> EDLLKNL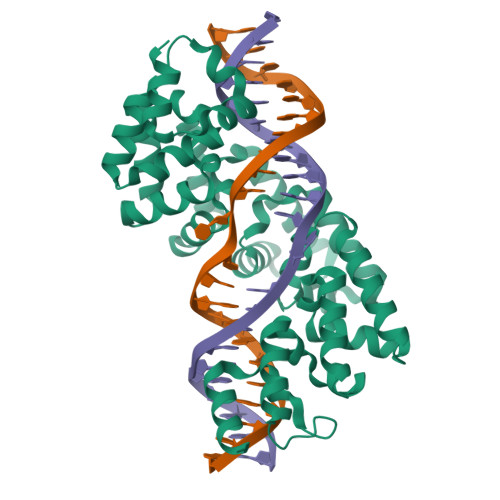LTMGVDIDMARKRQPGVFHRMITNEQDLKMFLLSKGASKEVIASIISRYPRAITRTPENLSKRWDLWRKIVTSDLEIVNILEASPESFFRSNNNLNLENNIKFLYSVGLTRKCLCRLLTNAPRTFSNSLDLNKQMVEFLQAAGLSLGHNDPADFVRKIIFKNPFILIQSTKRVKANIEFLRSTFNLNSEELLVLICGPGAEILDLSNDYARRSYANIKEKLFSLGCTEEEVQKFVLSYPDVIFLAEKKFNDKIDCLMEENISISQIIENPRVLDSSISTLKSRIKELVNAGCNLSTLNITLLSWSKKRYEAKLKKLS> SEEQVAQDTEEVFRSYVFYRHQQEQEAEGVAAPADPEMVTLPLQPSSTMGQVGRLLAIIGDDINRRYDSEFQTMLQHLQPTAENAYEYFTKIATSLFESGINWGRVVALLGFGYR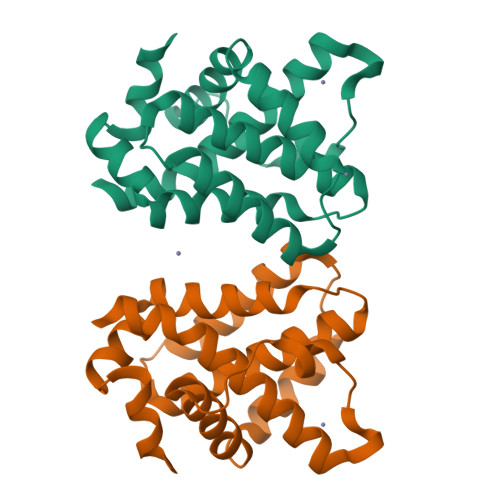LALHVYQHGLTGFLGQVTRFVVDFMLHHSIARWIAQRGGWVAALNLG>GAMGML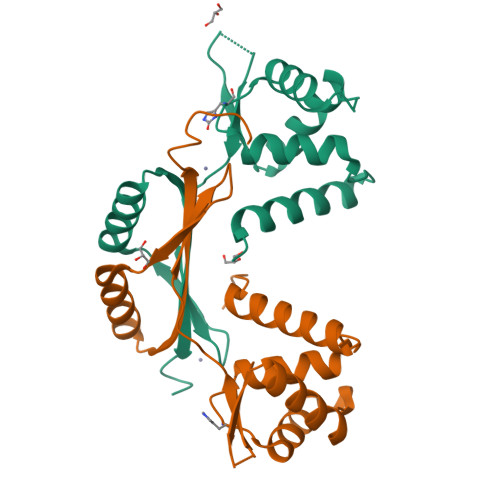IENVEYDVLLERFKKILRQGGLKYTKQREVLLKTLYHSDTHYTPESLYMEIKQAEPDLNVGIATVYRTLNLLEEAEMVTSISFGSAGKKYELANKPHHDHMICKNCGKIIEFENPIIERQQALIAKEHGFKLTGHLMQLYGVCGDCNNQKAKVKI[2x]> MIPLQHGLILAAILFVLGLTGLV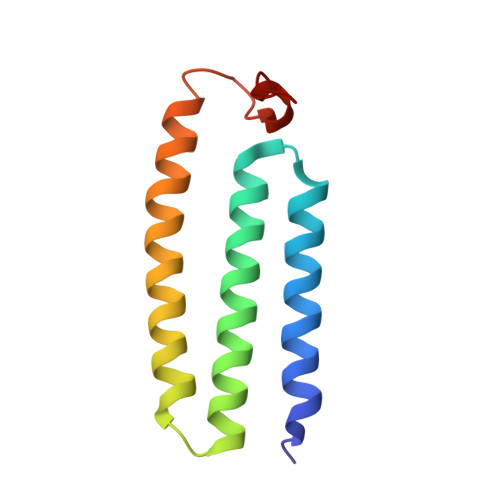IRRNLLFMLIGLEIMINASALAFVVAGSYWGQTDGQVMYILAISLAAAEASIGLALLLQLHRRRQNLNIDSVSEMRG>[2x]MGKVRNISGCVAVAHGVRLADVDVICSYPIRPYTGIMSELARMVADGELDAEFVHGEGEHAQLSVVYGASAAGARVFTGSSGVGVTYAMEVYSPISGERLPVQMAIADRTLDPPGDFGEEHTDAECCRDQGWIQGWASTPQEALDNTLIYYRVGEDQRVLLPQYACLDGYFVSHILGPVDIPDEAQVKEFLPPYKNHHVLDPRKPQIIGPQIEPAMGPPLQYQRYQAVKGVHKVLEEACDEFARIFGRKYDPYLDEYLTDDAEVIIFGQGAHMETAKAVARRLRNLGEKVGVARLRTFRPFPTEQIKERLSKFKAIGVLDVSANFGISCSGGVLLSELRAALYDYGDKVKTVGFVAGLGGEVVTHDEFYRMFQKLKEIAKTGKVEQTSYWIPFEL;>[2x]MSTKDLFAEPNLKQITVWARGVVMNKDARDIVVALTEAAAKEGKYVQAWENYVDLPDRIYVPVRAYARISSDPIESKYIYENETPDIVVLVEESLIKGVPILKGIRPGSTLVVNTKRSIDTILEFLGDTGNLAQIVTVDANSMAEAVMTLSGAEGATDATGIGAGIAAPIAGAVVKATGIVDVENLAAVVKNPAAMRRGYAEAQVRQLPPHEAVEEAAVSATELLRQMPFAGTVPSPVTENEGMVTGNWRIQRPIIDREACTECYTCWIYCPDSCITRTEEGPVFNMKYCKGCGLCTAVCPSGALTNVPELDFKD;>MLDRIASIKKAPDEEYYVPGHRTCAG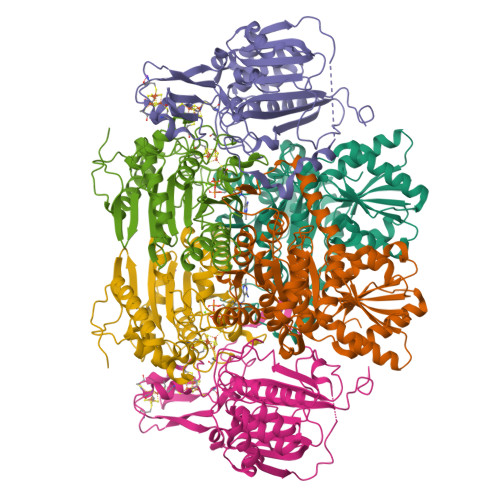CGPALTYRLVAKAAGPNTIFIGPTGCMYVANTSYGCGPWRVPWIHAQITNGGAVASGIEAAYKAMIRKKKTDAEFPNIIVMAGDGGAVDIGLQALSAMLYRGHDVLFICYDNESYANTGIQTSPTTPYGANTTFTPPGEVVPEGKKLFPKDNPKVIAHGHPELKYVATASIGWPVDLMNKVRKGLNQEGPAYIHIHAPCPKGWQFPADKTIEMAKLAVQTGMFQLYEYENGEYKLSVKVDKRKPVSEYMKLQKRFAHLKPEHIAKMQAFVDARCAEVGITVPVVASNA[2x]>[4x]MNTEALQSKFFSPLQKAMLPPNSFQGKVAFITGGGTGLGKGMTTLLSSLGAQCVIASRKMDVLKATAEQISSQTGNKVHAIQCDVRDPDMVQNTVSELIKVAGHPNIVINNAAGNFISPTERLSPNAWKTITDIVLNGTAFVTLEIGKQLIKAQKGAAFLSITTIYAETGSGFVVPSASAKAGVEAMSKSLAAEWGKYGMRFNVIQPGPIKTKGAFSRLDP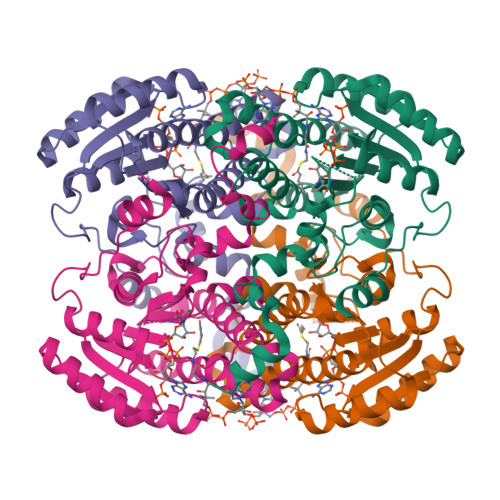TGTFEKEMIGRIPCGRLGTVEELANLAAFLCSDYASWINGAVIKFDGGEEVLISGEFNDLRKVTKEQWDTIEELIRKTKGS>LKDLFRYIWPKGNNKVRIRVLIALGLLISAKILNVQVPFFFKQTIDSMNIAWDDPTVALPAAIGLTILCYGVARFGSVLFGELRNAVFAKVAQNAIRTVSLQTFQHLMKLDLGWHLSRQTGGLTRAMDRGTKGISQVLTAMVFHIIPISFEISVVCGILTYQFGASFAAITFSTMLLYSIFTIKTTAWRTHFR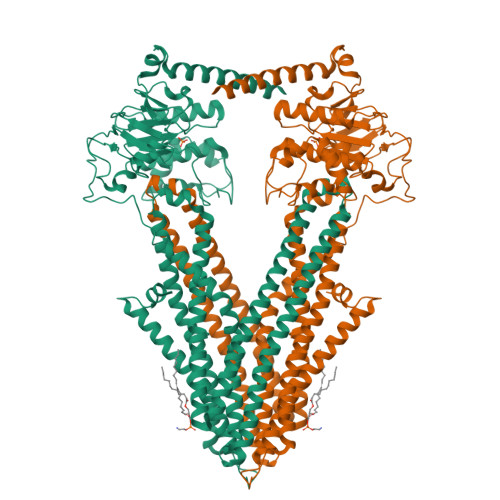RDANKADNKAASVALDSLINFEAVKYFNNEKYLADKYNGSLMNYRDSQIKVSQSLAFLNSGQNLIFTTALTAMMYMGCTGVIGGNLTVGDLVLINQLVFQLSVPLNFLGSVYRDLKQSLIDMETLFKLRKNEVKIKNAERPLMLPENVPYDITFENVTFGYHPDRKILKNASFTIPAGWKTAIVGSSGSGKSTILKLVFRFYDPESGRILINGRDIKEYDIDALRKVIGVVPQDTPLFNDTIWENVKFGRIDATDEEVITVVEKAQLAPLIKKLPQGFDTIVGERGLMISGGEKQRLAIARVLLKNARIMFFDEATSALDTHTEQALLRTIRDNFTSGSRTSVYIAHRLRTIADADKIIVLDNGRVREEGKHLELLAMPGSLYRELWTIQEDLDHLENELKDQQELWSHPQFEK[2x]> SFVKDFKPQALGDTNLFKPIKIGNNELLHRAVIPPLTRMRALHPGNIPNRDWAVEYYTQRAQRPGTMIITEGAFISPQAGGYDNAPGVWSEEQMVEWTKIFNAIHEKKSFVWVQLWVLGWAAFPDNLARDGLRYDSASDNVFMDAEQEAKAKKANNPQHSLTKDEIKQYIKEYVQAAKNSIAAGADGVEINSAHGYLLNQFLDPHSNTRTDEYGGSIENRARFTLEVVDALVEAIGHEKVGLRLSPYGVFNSMSGGAETGIVAQYAYVAGELEKRAKAGKRLAFVHLVEPRVTNPFLTEGEGEYEGGSNDFVYSIWKGPVIRAGNFALHPEVVREEVKDKRTLIGYGRFFISNPDLVDRLEKGLPLNKYDRDTFYQMSAHG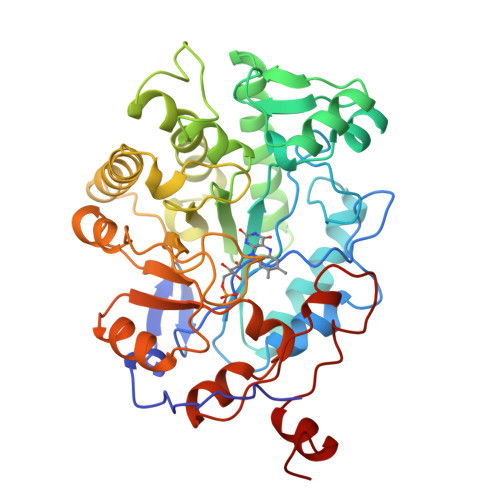YIDYPTYEEALKLGWDKS>SIPGQVADQAPLPSLAPMLEKVLPAVVSVRVEGTASQGQKIPEEFKKFFGDDLPDQPAQPFEGLGSGVIINASKGYVLTNNHVINQAQKISIQLNDGREFDAKLIGSDDQSDIALLQIQNPSKLTQIAIADSDKLRVGDFAVAVGNPFGLGQTATSGIVSALGRSGLNLEGLENFIQTDASINRGNSGGALLNLNGELIGINTAILAPGGGSVGIGFAIPSNMARTLAQQLIDFGEIKRGLLGIKGTEMSADIAKAFNLDVQRGAFVSEVLPGSGSAKAGV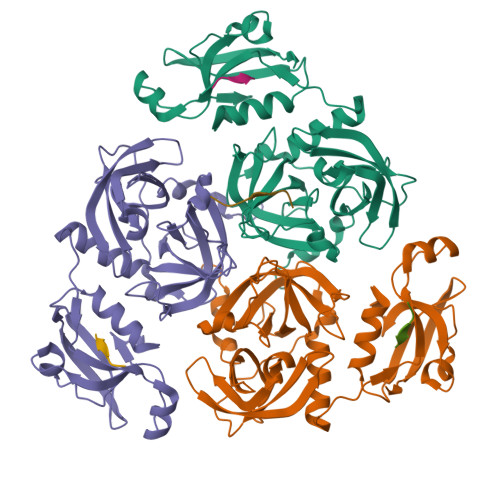KAGDIITSLNGKPLNSFAELRSRIATTEPGTKVKLGLLRNGKPLEVEVTLDTSTSSLEHHHHHH[12x]> PALISRLGALQQIIDDTPGIRLRTLSFDAARNALQLEI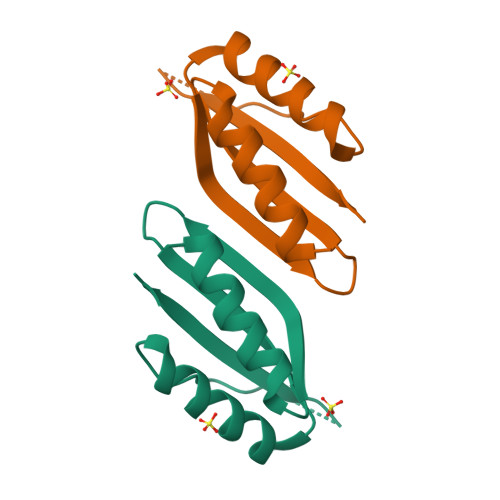SAVSSQALEQFSQRARARFRVQTGEMKPRADGIEGRLTLEG3,4,5-trimethoxybenzoic acid | 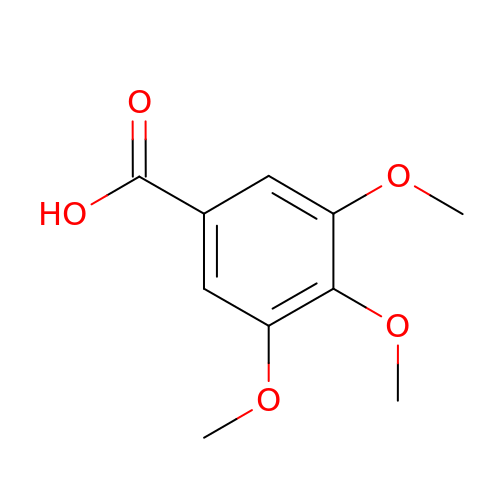C10 H12 O5 | SJSOFNCYXJUNBT-UHFFFAOYSA-N> GSHMKVKLDYEEVGACQKEVLITWDKKLLNCRAKIRCDMEDIHTLLKEGVPKSRRGEIWQFLALQYRLRHRLPNKQQPPDISYKELLKQLTAQQHAIL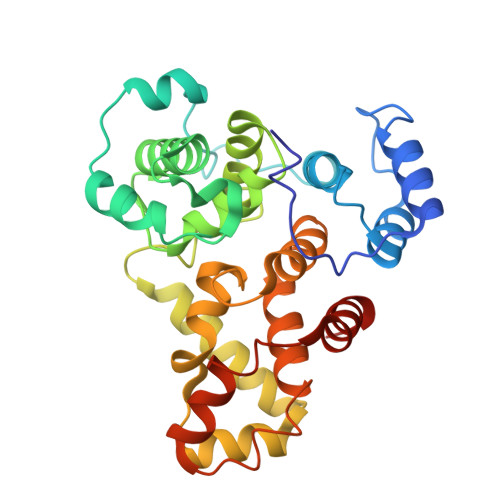VDLGRTFPTHPYFSVQLGPGQLSLFNLLKAYSLLDKEVGYCQGISFVAGVLLLHMSEEQAFEMLKFLMYDLGFRKQYRPDMMSLQIQMYQLSRLLHDYHRDLYNHLEENEISPSLYAAPWFLTLFASQFSLGFVARVFDIIFLQGTEVIFKVALSLLSSQETLIMECESFENIVEFLKNTLPDMNTSEMEKIITQVFEMDISK>MSKRPNFLVIVADDLGFSDIGAFGGEIATPNLDALAIAGLRLTDFHTTSAASPTRSMLLTGTDHHIAGLGTVAEALTPELEGKPGYEGHLNERVVALPELLREAGYQTLMAGKWHLGLKPEQTPHARGFERSFSLLPGAANHYGFEPPYDESTPRILKGTPALYVEDERYLDTLPEGFYSSDAF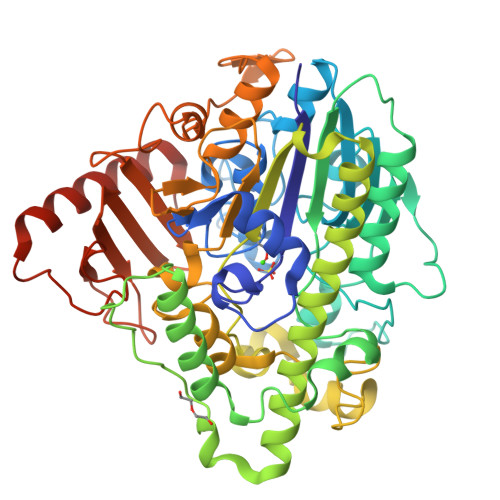GDKLLQYLKERDQSRPFFAYLPFSAPHWPLQAPREIVEKYRGRYDAGPEALRQERLARLKELGLVEADVEAHPVLALTREWEALEDEERAKSARAMEVYAAMVERMDWNIGRVVDYLRRQGELDNTFVLFMSDNGAEGALLEAFPKFGPDLLDFLDRHYDNSLENIGSANSYVWYGPRWAQAATAPSRLYKAFTTQGGIRVPALVRYPRLSRQGAISHAFATVMDVTPTLLDLAGVRHPGKRWRGREIAEPRGRSWLGWLSGETEAAHDENTVTGWGLFGMRAIRQGDWKAVYLPAPVGPATWQLYDLARDPGEIHDLADSQPGKLAELIEHWKRYVSDTGVVEGASPFLER[2x]>MFKAIVSAATLRDALDSVSVLVDECKIRLNEESLSIRAVDPANVGMVDLTLDAAAFESYEAHGGVIGVNLSRLEEVAGMAGAGDLIHLTLDEETRKLNIRIDGLSYTLALIDPDSIRQEPDIPDLDLAANIVLEGTHLDRGIKAADMVSDHIRLRVDGAEETFHIEAEGD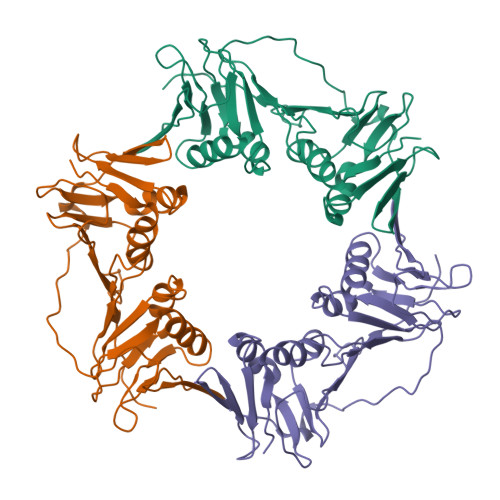TDDVDLSLPPADLISIEAGAADSLFSLDYLKDMNKAIPTDAEVTVELGEEFPVKLHYQIAEGMGTITYMLAPRIQSD[6x]>[4x]MKRMLINATQQEELRVALVDGQRLYDLDIESPGHEQKKANIYKGKITRIEPSLEAAFVDYGAERHGFLPLKEIAREYFPANYSAHGRPNIKDVLREGQEVIVQIDKEERGNKGAALTTFISLAGSYLVLMPNNPRAGGISRRIEGDDRTELKEALASLELPEGMGLIVRTAGVGKSAEALQWDLSFRLKHWEAIKKAAESRPAPFLIHQESNVIVRAFRDYLRQD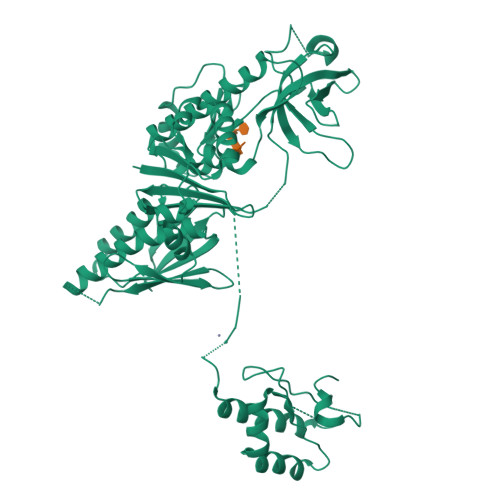IGEILIDNPKVLELARQHIAALGRPDFSSKIKLYTGEIPLFSHYQIESQIESAFQREVRLPSGGSIVIDSTEALTAIDINSARATRGGDIEETAFNTNLEAADEIARQLRLRDLGGLIVIDFIDMTPVRHQRAVENRLREAVRQDRARIQISHISRFGLLEMSRQRLSPSLGESSHHVCPRCSGTGTVRDNESLSLSILRLIEEEALKENTQEVHAIVPVPIASYLLNEKRSAVNAIETRQDGVRCVIVPNDQMETPHYHVLRVRKGEETPTLSYMLPKLHEEA phenazine-1,6-dicarboxylic acid 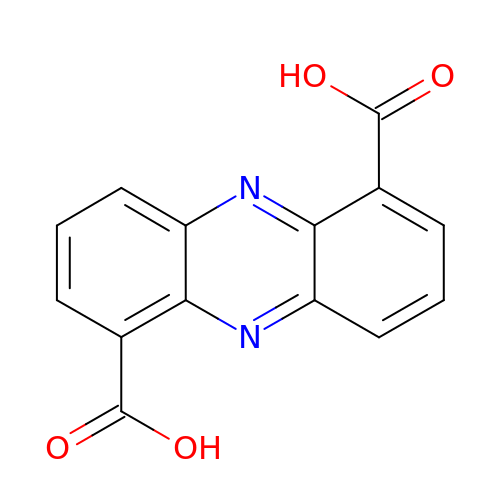| C14 H8 N2 O4 | MJALVONLCNWZHK-UHFFFAOYSA-N> MFRSAVLRSAAAATRTTIRSIPPAAAKKFAVAPVSRVTSFIPK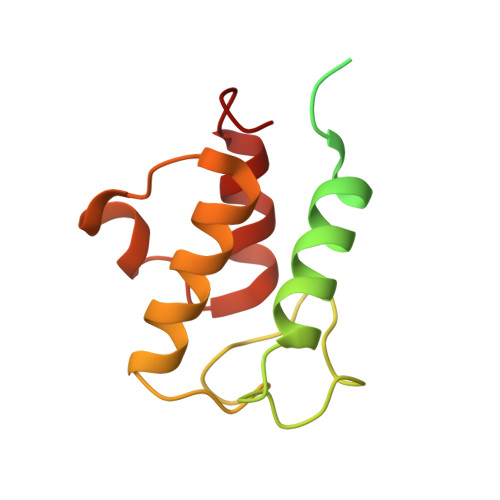TASWQVIRCYASNEGLQKVEVYERIKSLLAGFDKVNDPNNITETAHFANDLGLDSLDTVEVVMAIEEEFSIEIPDKDADQIHSVDKAIEYILRQPDAH> SRANDAPIVLLHGFTGWGREEMFGFKYWGGVRGDIEQWLNDNGYRTYTLAVGPLSSNWDRACEAYAQLVGGTVDYGAAHAAK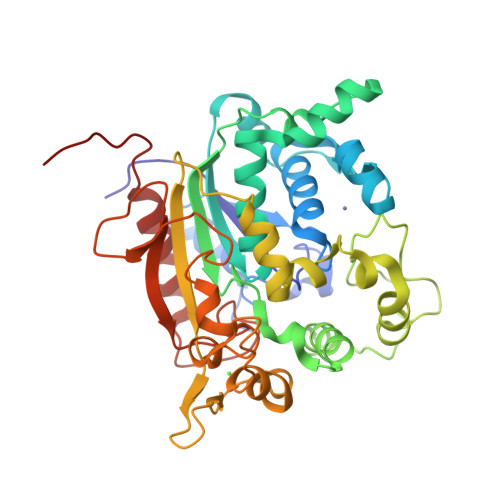HGHARFGRTYPGLLPELKRGGRIHIIAHSQGGQTARMLVSLLENGSQEEREYAKAHNVSLSPLFEGGHHFVLSVTTIATPHDGTTLVNMVDFTDRFFDFQKFVLKAAAVASNVPYTSQVYDFKLDQWGLRRQPGESFDQYFERLKRSPVWTSTDTARYDLSVPGAEKLNQWVKASPNTYYLSFATERTYRGALTGNYYPELGMNAFSAVVCAPFLGSYRNATLGIDDRWLENDGIVNAFSMNGPKRGSTDRIVPYDGTIKKGVWNDMGTYNVDHFEVIGVDPNPLFDIRAFYLRLAEQLASLQPHHHHHH> KVAP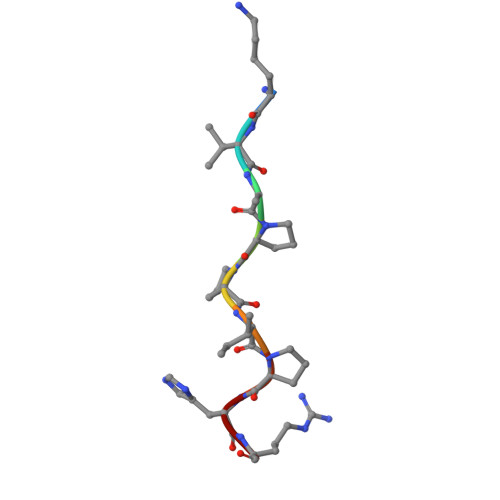PIPHR> MIATMTIAASLAISPAA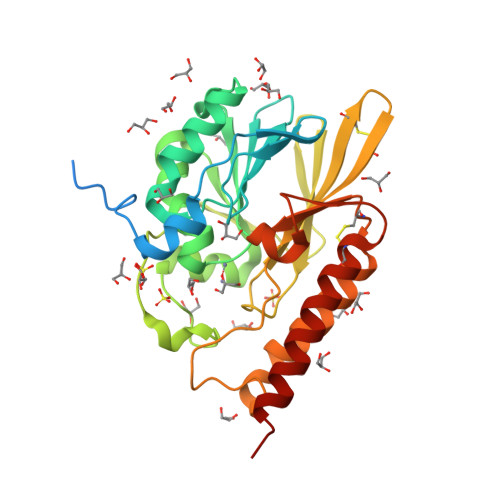AATGPEPEAMAAMDRAGGARASDDPLTRPMAVERAKEWLAPLPPERVFGNSYLVGFAGLSVALIDTGAGLVLIDGALPQAAPMILSNVRKLGFDPRDIKFILSTEPHYDHAGGIAALARDTGATVVASRRGAEGLRAGAHAKDDPQFDYGGAWPAVSRLRVMKDGEVLRIGRASITAHATPGHTMGSMTWSWNACEGKRCKAIVFASSLNPVSADRYRFTAPSSAPIVKGFEASYRRMGALKCDILISAHPDNAGAGRYGSGSGACRSYAERSRRLLAKRLAEERRETSK methyl 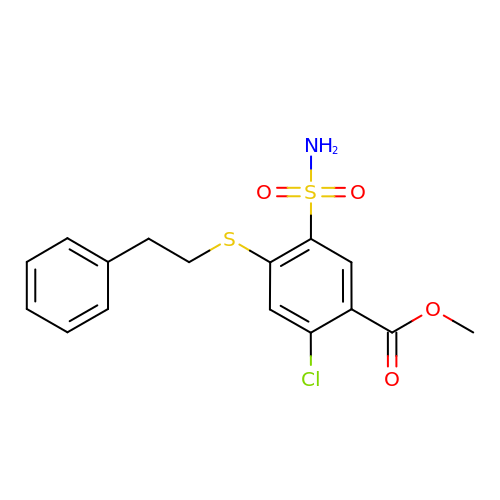2-chloranyl-4-(2-phenylethylsulfanyl)-5-sulfamoyl-benzoate | C16 H16 Cl N O4 S2 | KICJCRSMGGMWMV-UHFFFAOYSA-N> SNALNLPYDEHADAWTQVKKALAAGKRTHKPTLL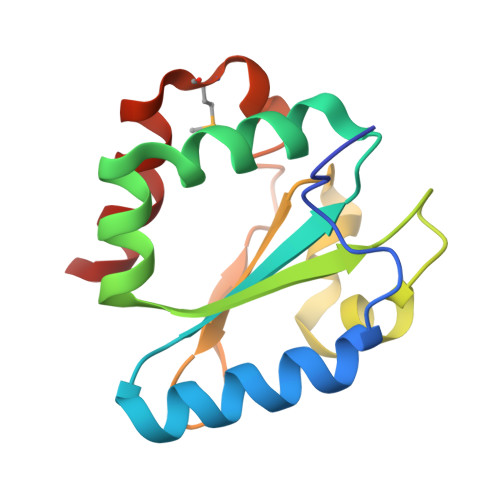VFGANWCTDCRALDKSLRNQKNTALIAKHFEVVKIDVGNFDRNLELSQAYGDPIQDGIPAVVVVNSDGKVRYTTKGGELANARKMSDQGIYDFFAKITE>[2x]GPHMAIHILTEKEDHATLHISFN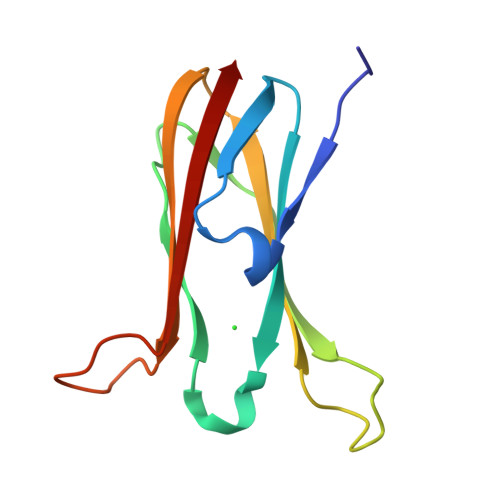DLIKIQLRTNPSTGYAWNIEYPTDTFSLSQDTIKAEPHPSGMVGFPSIREIQLKPLKVGTTTIKLGYSRPWEKGKEPLRSLTYSVVIR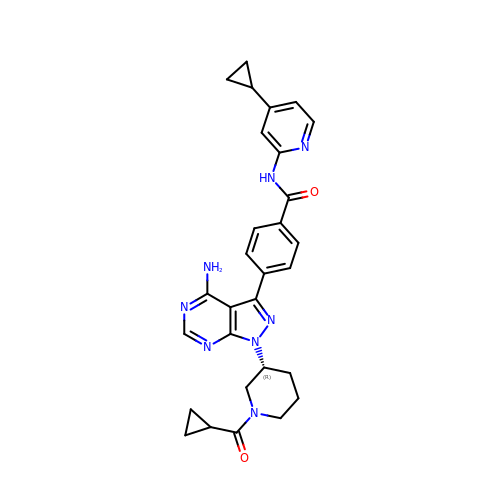4-{4-amino-1-[(3R)-1-(cyclopropanecarbonyl)piperidin-3-yl]-1H-pyrazolo[3,4-d]pyrimidin-3-yl}-N-(4-cyclopropylpyridin-2-yl)benzamide | C29 H30 N8 O2 | CTJGTZNFLORRFT-JOCHJYFZSA-N>SVKLAGNSSLCPVSGWAIYSKDNSVRIGSK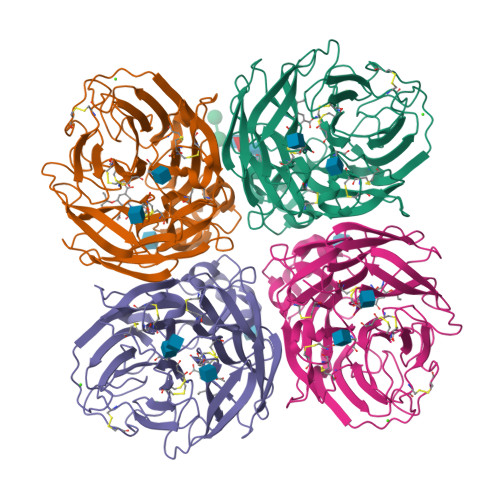GDVFVIREPFISCSPLECRTFFLTQGALLNDKHSNGTIKDRSPYRTLMSCPIGEVPSPYNSRFESVAWSASACHDGINWLTIGISGPDNGAVAVLKYNGIITDTIKSWRNNILRTQESECACVNGSCFTVMTDGPSNGQASYKIFRIEKGKIVKSVEMNAPNYYYEECSCYPDSSEITCVCRDNWHGSNRPWVSFNQNLEYQIGYICSGIFGDNPRPNDKTGSCGPVSSNGANGVKGFSFKYGNGVWIGRTKSISSRNGFEMIWDPNGWTGTDNNFSIKQDIVGINEWSGYSGSFVQHPELTGLDCIRPCFWVELIRGRPKENTIWTSGSSISFCGVNSDTVGWSWPDGAELPFTIDK[4x]> MKDYDELLKYYELYETIGTGGFAKVKLACHVLTGEMVAIKIMDKNALGSDLPRVKTEIDALKSLRHQHICQLYHVLETKNKIFMVLEYCPGGELFDYIISQDRLSEEETRVVFRQILSAVAYVHSQGYAHRDLKPENLLFDENHKLKLIDFGLCAKPKGNKDYHLQECCGSLAYAAPELIQGKSYLGSEADVWSMGILLYVLMCGFLPFDDDNVMALYKKIMRGKYEVPKWLSPSSILLLQQMLQVDPKKRISMRNLLNHPWVMQDYSCPVEWQSKTPLTHLDEDCVTELSVHHRSSRQTMEDLISSWQYDHLTATYLLLLAKKARLEHHHHHH

Murine protein serine/threonine kinase 38 (MPK38) is the murine orthologue of human maternal embryonic leucine-zipper kinase (MELK), which belongs to the SNF1/AMPK family. MPK38 consecutively comprises a kinase domain (KD), a ubiquitin-associated (UBA) domain, a TP dipeptide-rich domain and a kinase-associated 1 (KA1) domain. Activation of MPK38 requires the extended sequence (ExS) containing the ubiquitin-associated (UBA) linker and UBA domain and phosphorylation of the activation loop. MELK is considered to be a promising drug target for anticancer therapy because overexpression and hyperactivation of MELK is correlated with several human cancers.

However, the activation mechanism of MPK38 is unknown. This paper reports the crystal structure of MPK38 (T167E), which mimics a phosphorylated state of the activation loop, in complex with AMP-PNP. In MPK38, Thr167 is substituted by Glu to mimic the phosphorylated state of the activation loop. The overall structure of MPK38 (T167E) shows the KD and ExS, which contain the UBA linker and the UBA domain. The KD of MPK38 (T167E) adopts the classical bilobar protein kinase fold, which consists of an N-terminal lobe (N-lobe; residues 1–91) and a C-terminal lobe (C-lobe; residues 94–263). The AMP-PNP, which is an analogue of ATP, is positioned in the ATP-binding pocket. The UBA domain of MPK38 is a small globular domain that contains three short helices (α1–α3) and binds to the back of the N-lobe. In MPK38, Thr277 and Leu279 of the UBA linker modulate the αC helix from the ‘out’ to the ‘in’ position via a strong van der Waals interaction with Arg65 of the αC helix and an additional hydrogen bond in the vicinity; in detail, the O atom of the hydroxyl group of Thr277 interacts with the Cγ and N∊ atoms of Arg65 at distances of 3.4 and 3.6 Å, respectively. Additionally, the phosphorylation-mimic mutation in the activation loop triggered reorganization of the activation loop and the interlobar cleft into a more closed conformation. The activation loop in our MPK38 structure is partially stabilized because the glutamate does not completely mimic a phosphorylated state and the interactions with the surrounding residues (such as Arg131 of the catalytic loop) are not stable.>MADPRPDPDELARRA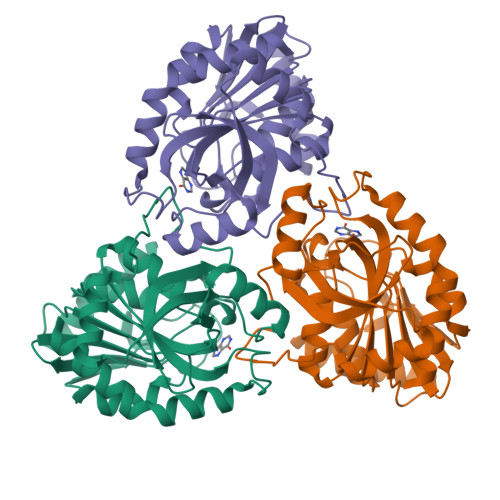AQVIADRTGIGEHDVAVVLGSGWLPAVAALGSPTTVLPQAELPGFVPPTAAGHAGELLSVPIGAHRVLVLAGRIHAYEGHDLRYVVHPVRAARAAGAQIMVLTNAAGGLRADLQVGQPVLISDHLNLTARSPLVGGEFVDLTDAYSPRLRELARQSDPQLAEGVYAGLPGPHYETPAEIRMLQTLGADLVGMSTVHETIAARAAGAEVLGVSLVTNLAAGITGEPLSHAEVLAAGAASATRMGALLADVIARF[2x]TRIAP1 (yeast Mdm35) and PRELI (yeast Ups) proteins reside within the IMS where they regulate phospholipid metabolism. Thus, lipid transfer proteins of the Ups/PRELI-family shuttle phospholipids across the IMS in a phospholipid specific manner. The partner protein TRIAP1/Mdm35 has an important role in mitochondrial import and folding of the PRELI domain as well modulating its membrane affinity. The Ups/PRELI lipid transfer proteins are widely conserved in eukaryotes and can be classified into two subfamilies by sequence similarity (Ups1/PRELID1 and Ups2/PRELID3).

Similarly, the human homologue PRELID1–TRIAP1 mediate PA transfer within the cardiolipin synthetic pathway. A construct of PRELID1 in which an unstructured region from residue 173 was omitted and Cys112 and 115 were substituted for serine residues facilitated the best soluble protein production (PRELID11–173) with no effect on activity. The structures of PRELID11–173–TRIAP1 and PRELID3b–TRIAP1 were solved by molecular replacement and refined to 1.98 and 2.91 Å resolution, respectively. In contrast for PRELID11–173, the Ω loop and the C-terminal α3 helix are much more closed than PRELID3b. PRELID11–173 exhibits the most closed of all the structures while the structure of PRELID3b displays the most open entrance to the lipid binding cavity, and this likely contributes to its ability to readily accept the larger headgroup of PS. Mass spectrometry (MS) identified that a fatty acid, likely an endogenous E. coli lipid molecule, was bound to PRELID1 and the abundant E. coli phospholipid phosphatidylglycerol (PG) was present in PRELID3b. While efficiently mediating the transfer of PA, PRELID1 showed a low PS transfer activity, similar to Ups114. K58 points into the lipid binding cavity of the PRELI domain and together with R25 make a specific electrostatic interaction with the negatively charged phosphomonoester of PA. K58 was notable in the PA release pathway as it maintained contact with the PA headgroup in the secondary site.

>DKMNSVGEACTDMKREYDQCFNRWFAEKFLKGDSSGDPCTDLFKRYQQCVQKAIKEKEIPIEGLEFMGH[2x];>HHHHHHSDQMVKYFLGQSVLRSSWDQVFAAFWQRYPNPYSKHVLTEDIVHREVTPDQKLLSRRLLTKTNRMPRWAERLFPANVAHSVYVLEDSIVDPQNQTMTTFTWNINHARLMVVEERSVYSVNSDNSGWTEIRREAWVSSSLFGVSRAVQEFGLARFKSNVTKTMKGFEYILAKLQGEA[2x]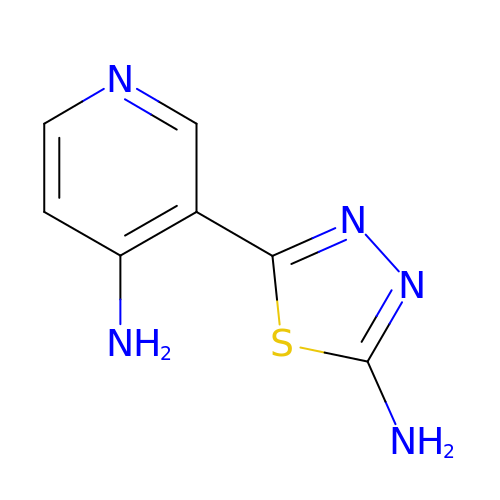3-(5-amino-1,3,4-thiadiazol-2-yl)pyridin-4-amine | C7 H7 N5 S | MNHIQWZHQXNGMA-UHFFFAOYSA-N> NQKCSGNPRRYNGKSCASTTNYHDSHKGACGCGPASGDAQFGWNAGSFVAAASQMYFDSGNKGWCGQHCGQCIKLTTTGGYVPGQGGPVREGLSKTFMITNLCPNIYPNQDWCNQGSQYGGHNKYGYELHLDLENGRSQVTGMGWNNPETTWEVVNCDS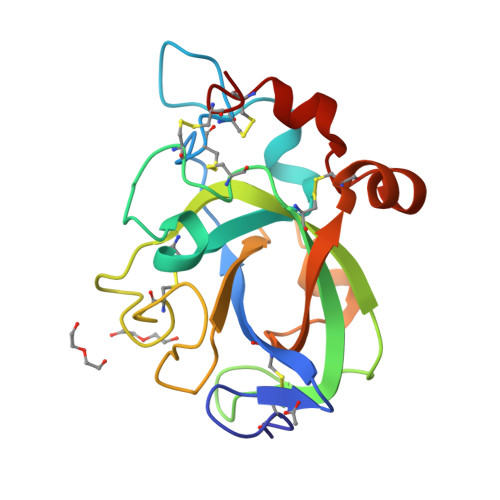EHNHDHRTPSNSMYGQCQCAHQ>MHHHHHHGGGGGMPASFERKLITRDALAAMRASLPAPVVFTNGVFDILHRGHVSYLADAKALGACLIVGVNSDASVRMLGKGDDRPINVQEDRMALLAALECVDWVVGFDEK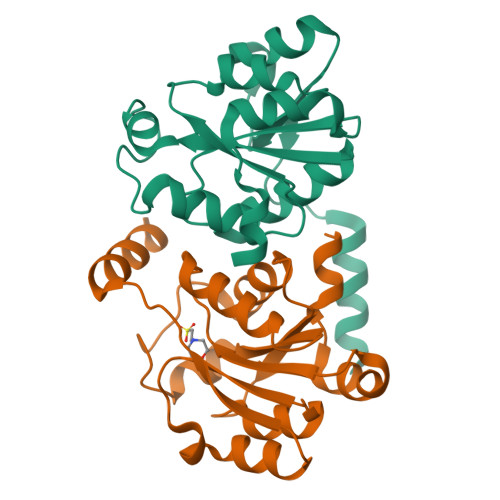TPVSLIEAVHPDILVKGGDYDMDALPESALVRGWGGRALAIPFEHDRSTTALLKKVRAQSR[4x]> MQPFDSGHDDLVHDVVYDFYGRHVATCSSDQHIKVFKLDKDTSNWELSDSWRAHDSSIVAIDWASPEYGRIIASASYDKTVKLWEEDPDQEECSGRRWNKLCTLNDSKGSLYSVKFAPAHLGLKLACLGNDGILRLYDALEPSDLRSWTLTSEMKVLSIPPANHLQSDFCLSWCPSRFSPEKLAVSALEQAIIYQRGKDGKLHVAAKLPGHKSLIRSISWAPSIGRWYQLIATGCKDGRIRIFKITEKNLQVELLSEHDDHNGEVWSVSWNLTGTILSSAGDDGKV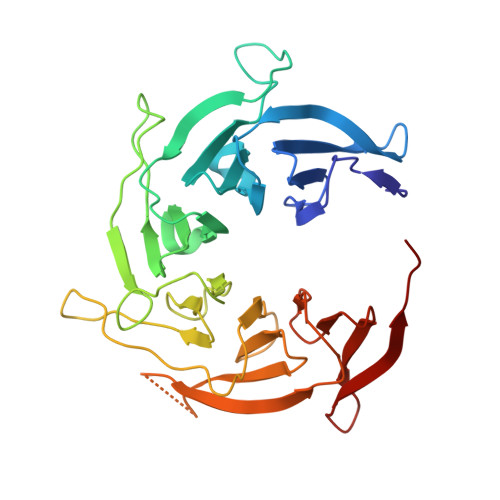RLWKATYSNEFKCMSVITAQQ>[4x]GSSHHHHHHSSGENLYFQGHMTCPFADPAALYSRQDTTSGQSPLAAYEVDDSTGYLTSDVGGPIQDQTSLKAGIRGPTLLEDFMFRQKIQHFDHERVPERAVHARGAGAHGTFTSYADWSNITAASFLNATGKQTPVFVRFSTAAGSRGSADTARDVHGFATRFYTDEGNFDIVGNNIPVFFIQDAIQFPDLIHSVKPRPDNEIPQAATAHDSAWDFFSQQPSTMHTLFWAMSGHGIPRSYRHMDGFGVHTFRFVKDDGSSKLIKWHFKSRQGKASLVWEEAQVLSGKNADFHRQDLWDAIESGNGPEWDVCVQIVDESQAQAFGFDLLDPTKIIPEEYAPLTKLGLLKLDRNPTNYFAETEQVMFQPGHIVRGIDFTEDP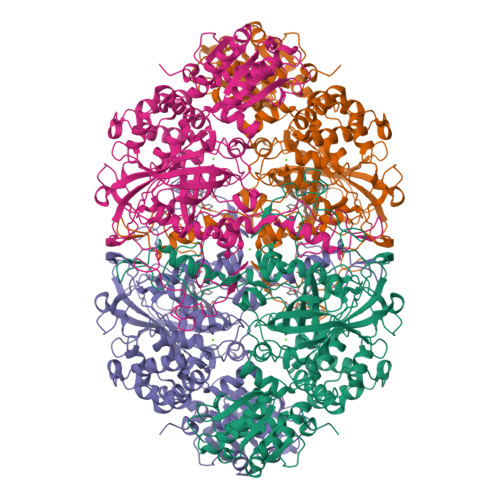LLQGRLFSYLDTQLNRNGGPNFEQLPINMPRVPIHNNNRDGAGQMFIHRNKYPYTPNTLNSGYPRQANQNAGRGFFTAPGRTASGALVREVSPTFNDHWSQPRLFFNSLTPVEQQFLVNAMRFEISLVKSEEVKKNVLTQLNRVSHDVAVRVAAAIGLGAPDADDTYYHNNKTAGVSIVGSGPLPTIKTLRVGILATTSESSALDQAAQLRTRLEKDGLVVTVVAETLREGVDQTYSTADATGFDGVVVVDGAAALFASTASSPLFPTGRPLQIFVDAYRWGKPVGVCGGKSSEVLDAADVPEDGDGVYSEESVDMFVEEFEKGLATFRFTDRFALDS>[4x]MDWRHKAVCRDEDPELFFPVGNSGPALAQIADAKLVCNRCPVTTECLSWALNTGQDSGVW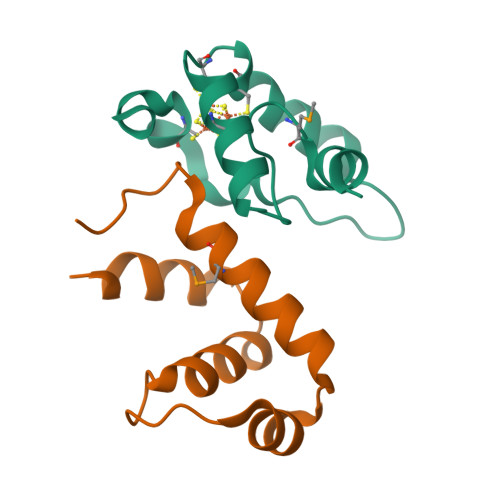GGMSEDERRALKRRNA;>[4x]MAHHHHHHAREPISLDQTIGDEGDSQLGDFIEDSEAVVAVDAVSFTLLQDQLQSVLDTLSEREAGVVRLRFGLTDGQPRTLDEIGQVYGVTRERIRQIESKTMSKLRHPSRSQVLRDYLD>[2x]AESTLGAAAAQSGRYFGTAIASGKLGDSAYTTIASREFNMVTAENEMKIDATEPQRGQFNFSAGDRVYNWAVQNGKQVRGHTLAWHSAQPGWMQSLSGSTLRQAMIDHINGVMGHYKGKIAQWDVVNEAFSDDGS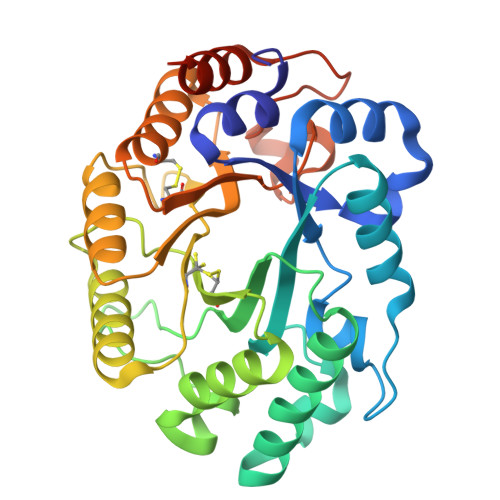GGRRDSNLQRTGNDWIEVAFRTARAADPAAKLCYNDYNIENWTWAKTQGVYNMVRDFKQRGVPIDCVGFQSHFNSGSPYNSNFRTTLQNFAALGVDVAITELDIQGASSSTYAAVTNDCLAVSRCLGITVWGVRDTDSWASGDTPLLFNGDGSKKAAYTAVLNALNGGGSRSHHHHHH> MDSRLQEIRERQKLRRQLLAQQLGAESADSIGAVLNSKDEQREIAETRETCRASYDTSAPNAKRKYLDEGETDEDKMEEYKDELEMQQDEENLPYEEEIYKDSSTFLKGTQSLNPHNDYCQHFVDTGHRPQNFIRDVGLADRFEEYPKLRELIRLKDELIAKSNTPPMYLQADIEAFDIRELTPKFDVILLEPPLEEYYRETGITANEKCWTWDDIMKLEIDEIAAPRSFIFLWCGSGEGLDLGRVCLRKWGYRRCEDICWIKTNKNNPGKTKTLDPKAVFQRTKEHCLMGIKGTVKRSTDGDFIHANVDIDLIITEEPEIGNIEKPVEI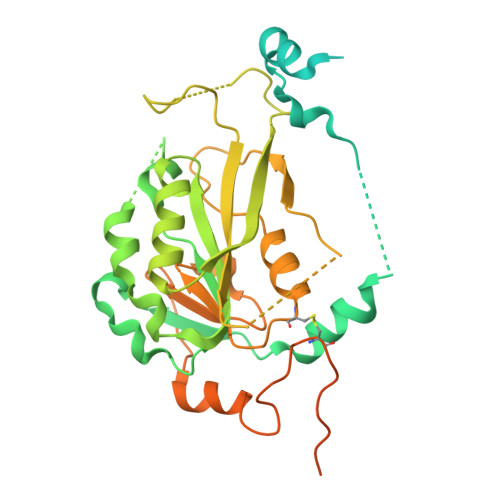FHIIEHFCLGRRRLHLFGRDSTIRPGWLTVGPTLTNSNYNAETYASYFSAPNSYLTGCTEEIERLRPKSPPPKSKSDRGGGAPRGGGRGGTSAGRGRERNRSNFRGERGGFRGGRGGAHRGGFPPR> SNAGVSDVELRVALPDGTTVTVRVKKNSTTDQVYQAIAAKVGMDSTTVNYFALFEVISHSFVRKLAPNEFPHKLYIQNYTSAVPGTCLTIRKWLFTTEEEILLNDNDLAVTYFFHQAVDDVKKGYIKAEEKSYQLQKLYEQRKMVMYLNMLRTCEGYNEIIFPHCACDSRRKGHVITAISITHFKLHACTEEGQLENQVIAFEWDEMQRWDTDEEGMAFCF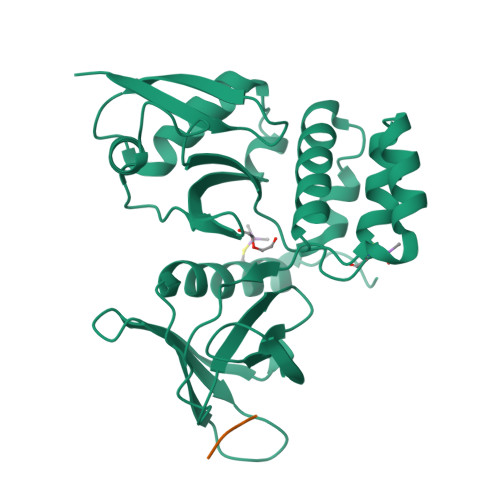EYARGEKKPRWVKIFTPYFNYMHECFERVFCELKWRKEEY;> SIFDDDMDDIFSSG> QQVGTSQAEVHPSMTWQSCTAGGSCTTNNGKVVIDANWRWVHKVGDYTNCYTGNTWDTTICPDDATCASNCALEGANYESTYGVTASGNSLRLNFVTTSQQKNIGSRLYMMKDDSTYEMFKLLNQEFTFDVDVSNLPCGLNGALYFVAMDADGGMSKYPTNKAGAKYGTGYCDSQCPRDLKFINGQANVEGWQPSSNDANAGTG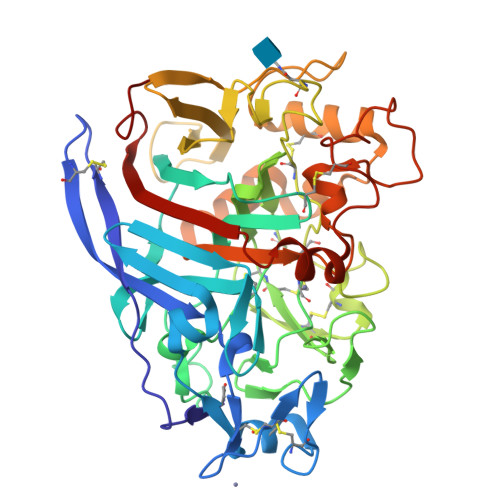NHGSCCAEMDIWEANSISTAFTPHPCDTPGQVMCTGDACGGTYSSDRYGGTCDPDGCDFNSFRQGNKTFYGPGMTVDTKSKFTVVTQFITDDGTSSGTLKEIKRFYVQNGKVIPNSESTWTGVSGNSITTEYCTAQKSLFQDQNVFEKHGGLEGMGAALAQGMVLVMSLWDDHSANMLWLDSNYPTTASSTTPGVARGTCDISSGVPADVEANHPDAYVVYSNIKVGPIGSTFNSG>[2x]GHMSRRGLEREGGKPVSSDAKGLKRVDVRLKWDPSPWDRPPHHLDIIATTYAADAPHGRPVYVVQFDKRSPDGT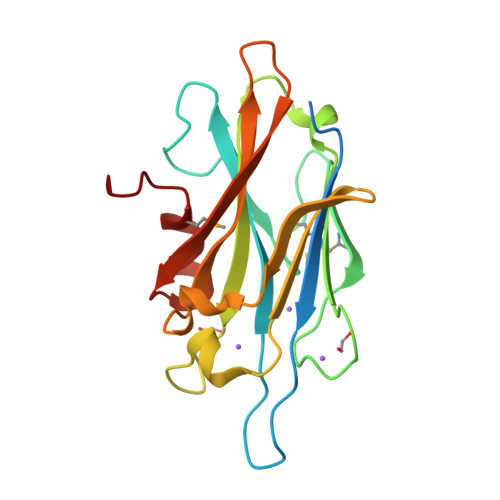INMSRHSRTGQGFGFVEEMTFELDRLSPSIARVIVGVAIHQDNGHKTFDDVSNTGVVVAEGYRELLTDGFERVAGATAATVAEFTRNASGAWEFREAVRGFDSDPVLFATEMGSAPRPGS>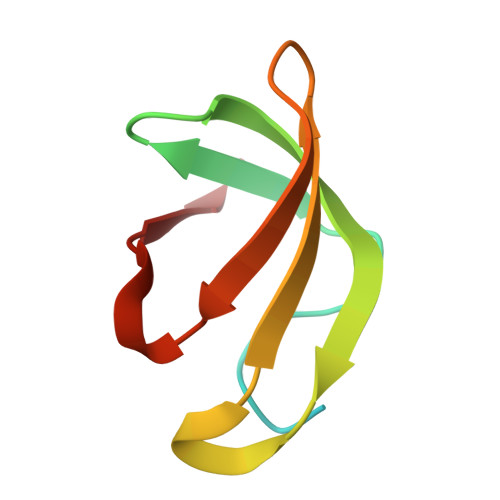 AMDVSHQRMGTPMVENDSGYKLGQRVRHAKFGEGTIVNMEGSGEHSRLQVAFQGQGIKWLVAAYARLESV> NYCNQMMKSRNLTKDRCKPVNTFVHESLADVQAVCSQKNVACKNGQTNCYQSYSTMSITDCRETGSSKYPN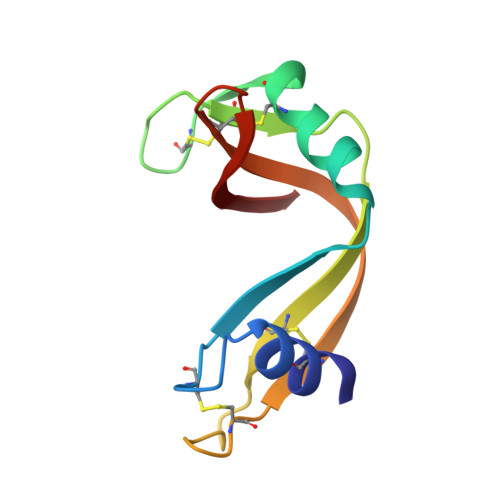CAYKTTQANKHIIVACEGNPYVPVHFDASV>SPSPWDFLGRVLQFQHGDHKRWWDVLAPVFGISMASIGYKLDVQYRHLLVLYDAVIPNMGPFPNSNASNITWTSPFPPGPLEASVNYQAGESSMFRFTIEPVGPHAGTPADPVNELAAKQLMQRLGQLQPGGVDSTMFDHFYPLLCVDGPEARRQWDSIAHIYHKCHTVTALDMQRSAACTLKTYFPPLLRSTIMNTSMVDIMFDAVESFRKQSGLYFDYTKIKEFMSEEKTHETMMVDRSYLSFDCLDPAKSRIKIYTEAKVKTLEEAYSFWSLGGRLSGPEIDYGFKIVSQMWDAIYSKELPGGKQRENNHIQINWEMSAKDSSVAPKLYLTVIEDYDAYVSSAIVDLFTGLGWAAHVQTHKKIEKEAYPMCDANPQSTHAYVWIS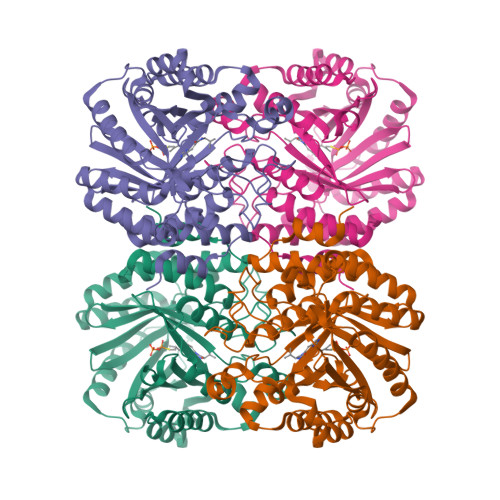LAYKKTGPYITVYTNPGASILE[4x]>HRILIERQEKSDTNFKEFVIKKLQKNCQCSPAKAKNMILGFLPVLQWLPKYDLKKNILGDVMSGLIVGILLVPQSIAYSLLAGQEPVYGLYTSFFASIIYFLLGTSRHISVGIFGVLCLMIGETVDRELQKAGYDNAHSAPSLGMVSNGSTLLNHTSDRICDKSCYAIMVGSTVTFIAGVYQVAMGFFQVGFVSVYLSDALLSGFVTGASFTILTSQAKYLLGLNLPRTNGVGSLITTWIHVFRNIHKTNLCDLITSLLCLLVLLPTKELNEHFKSKLKAPIPIELVVVVAATLASHFGKLHENYNSSIAGHIPTGFMPPKVPEWNLIPSVAVDAIAISIIGFAITVSLSEMFAKKHGYTVKANQEMYAIGFCNIIPSFFHCFTTSAALAKTLVKESTGCHTQLSGVVTALVLLLVLLVIAPLFYSLQKSVLGVITIVNLRGALRKFRDLPKMWSISRMDTVIWFVTMLSSALLSTEIGLLVGVCFSIFCVILRTQKPKSSLLGLVEESEVFESVSAYKNLQIKPGIKIFRFVAPLYYINKECFKSALYKQTVNPILIKVAWKKAAKRKIKEKVVTLGGIQDEMSVQLSHDPLELHTIVIDCSAIQFLDTAGIHTLKEVRRDYEAIGIQVLLAQCNPTVRDSLTNGEYCKKEEENLLFYSVYEAMAFAEVSKN[2x]

SLC26A2 is a vital solute carrier responsible for transporting essential nutritional ions, including sulfate, within the human body. SLC26A2 is known to function as an electroneutral anion exchanger, facilitating the exchange of various substrates such as SO42− and C2O42− for Cl−, hydroxide (OH−), or even with each other. Like its homologs, SLC26A2 forms a domain-swapped homodimer. Each protomer of SLC26A2 can be divided into three regions: the N-terminal region (residues 1–104) comprising a few flexible cytosolic helices and loops, the transmembrane domain (TMD, residues 105–540) with 14 transmembrane helices (TMs), and the C-terminal cytosolic sulfate transporter and anti-sigma factor antagonist domain (STAS, residues 541–739).

In addition to its known transport of SO42− and Cl−, SLC26A2 is also capable of C2O42− transport. We determined the structure of SLC26A2-C2O42− without NaCl to an overall resolution of ~3 Å. Surprisingly, we found no experimental density for C2O42− in the canonical substrate-binding pocket between TM3 and TM10. Instead, we found weak densities outside the pocket, in the core and gate domains interface between TM5 and TM12, which could accommodate a C2O42− molecule. Our model shows that the C2O42− substrate is likely stabilized via interactions with the side chains of adjacent Ser residues, as well as backbone carbonyls from L253. We mutated the Ser residues and carried out the cellular transport assay. The result shows a ~ 40% reduction in transport efficiency, confirming the importance of these Ser residues for C2O42− translocation. In addition, we performed molecular dynamics simulations to probe the dynamics between SLC26A2 and the C2O42−. The result showed that C2O42− remains bound for ~65 ± 4 % of the time. Notably, in all simulations, the C2O42− molecule does not enter the exact binding pocket that accommodates Cl− and SO42−, implying that the substrates’ transport pathways might not be exactly the same.2-[(2',3',4'-TRIFLUOROBIPHENYL-2-YL)OXY]ETHANOL | C14 H11 F3 O2 | 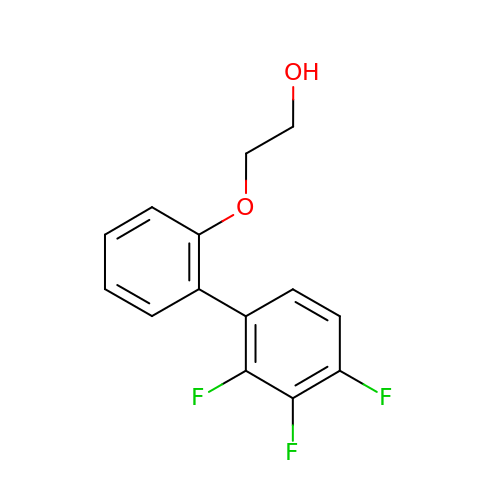AGXPXFPIOHNDAN-UHFFFAOYSA-N MEILB2 (meiotic localiser of BRCA2; also known as HSF2BP) was recently identified as a meiosis-specific interacting partner of BRCA2. BRME1 (BRCA2 and MEILB2-associating protein 1; also known as MEIOK21, MMER, C19ORF57 and 4930432K21Rik) was then identified as a meiosis-specific binding partner of MEILB2. The particular adaptations of meiotic recombination require several additional meiosis-specific components. These include the MEILB2–BRME1 complex, which binds directly to BRCA2 and is essential for the correct localisation of RAD51 and DMC1 recombinases to meiotic DSBs.

Here, we identified an optimised construct for crystallography, which includes the α1 helix and the beginning of the α2 helix of MEILB2 (amino-acids 22–81; herein referred to as MEILB2α) and the core of BRME1’s MBD (amino-acids 540–578; herein referred to as BRME1MBD). Crystals of this MEILB2α–BRME1MBD complex diffracted to a resolution limit of 1.50 Å, enabling structure solution by molecular replacement of ideal helical fragments using ARCIMBOLDO_LITE45. Thus, the overall structure of MEILB2α–BRME1MBD can be described as a parallel 2:2 α/β-coiled-coil, where an N-terminal MEILB2 β-cap is followed by a MEILB2α1–BRME1 four-helical bundle that transitions via a kink into a C-terminal MEILB2 α2 dimeric coiled-coil. The MEILB2α–BRME1MBD structure contains an unusual β-cap at its N-terminal tip. This consists of an anti-parallel two-stranded β-sheet, which is formed by the N-terminal ends of MEILB2 chains, and is orientated perpendicular to the helical axis. The β-cap binds together the N-termini of the two α1 helices of the four-helical bundle, so likely prevents the fraying apart of helical ends that typically occurs within coiled-coil structures. At this point, there is a slight ‘kink’ in the MEILB2 chains, between α1 and α2 helices, where L50 and N51 adopt non-helical conformations due to a single amino-acid insertion into the heptad repeats. The hydrophobic core of the four-helical bundle comprises highly conserved BRME1 amino acids V548, L555 and I562, which occupy the ‘a’ positions within the heptad repeats. Thus, DNA binding is mediated by the rigid β-cap at the N-terminal tip of the MEILB2–BRME1MBD structure.

>GSMEEFVKVRKKDLERLTTEVMQIRDFLPRILNGELLESFQKLKMVEKNLERKEQELEQLIMD[2x];>[2x]GSMRMQDATDTVRGLVVELSGLNRLIMSTHRDLEAFKR We focus on AMGs that potentially encode chitosanase enzymes that metabolize chitin – a common carbon polymer. One expressed protein showing endo-chitosanase activity (V-Csn) is crystalized and structurally characterized at ultra-high resolution, thus representing the structure of a soil viral AMG product. The structure consisted of two non-contiguous structural domains. Our rigorous analyses not only resulted in a crystal structure of a soil viral AMG product, but also enabled us to propose the mode of action of this previously uncharacterized chitosanase enzyme in the GH75 family of glycosyl hydrolases.

Co-crystallization of both mutant proteins with chitohexaose (a β-(1-4)-linked polymer of six D-glucosamine (GlcN) residues) gave a complex with the E157Q mutant only. The substrate was located in the interdomain cleft, with three of the six GlcN residues (hereinafter named GlcN-1, GlcN-2 and GlcN-3) visible in Fo-Fc electron density, oriented such that GlcN-1 is the reducing end. The GlcN-2 and GlcN-3 residues are in a standard chair conformation, however, the density for the first observed residue (GlcN-1) suggested a distorted boat conformation. The GlcN-1 residue is anchored by a single hydrogen bond between the O6 atom and the side chain of Q157. The central GlcN residue (GlcN-2) makes hydrogen bonding interactions with the side chains of D148 and D36 via its free amine, along with a third to the backbone carbonyl oxygen of A90 from Domain-2. The GlcN-3 residue makes a hydrogen bonding interaction with the carbonyl oxygen of T91 via the O6 atom, and another to a water molecule. Although some additional Fo-Fc density was observed at the non-reducing end of GlcN-3 (the O4 atom), the sparsity of the density did not allow for a fourth GlcN to be modelled. The location of the trisaccharide fragment and the interactions it makes with the protein suggests that residues D36 and D148 form the −2 subsite and play a key role in binding and orienting the substrate (in this case via the GlcN-2 residue). The E157 residue represents the −1 subsite and may serve as the nucleophilic group responsible for bond cleavage, assuming that hydrolysis occurred at the reducing end of GlcN-1. A loop in V-Csn Domain-2 (residues Ala90 and Thr91) is involved in formation of the −2 and −3 subsites and would be expected to correctly orient this end of the chitosan substrate for optimal positioning of the −1/+1 cleavage site.

> HMSELSEIDSVAGVTIYSVDGEPKSFVYKAGFAIDADGAPNAYAPNNGGTDFTANGGDDQGGDWWGGPVDAEGYPIKQKIFDPFPGYYVSATAHFNPAYSEDSPYRYIDSNSIPFIVLPGNHSNGAKLGDVALVYNEKTGDNCYAIYGDVGPSSKIGQGSVRLAQALKIDDNPKAGGTESRIVVTLVFPGSVGKWETPKRWFSHANQLTKAWGGLSRLKTLSDQL> MGGIMQLVSTGYQDVFLTGDPTRSLWKRIMARKTNFAIESIETVFDVLYGSTSFINIKKAGDLLKSCVLEITMKRTSTESFYPAEQFIKSLTLLIGDQEVEKIQDFPTWSRVHDELFNDTEM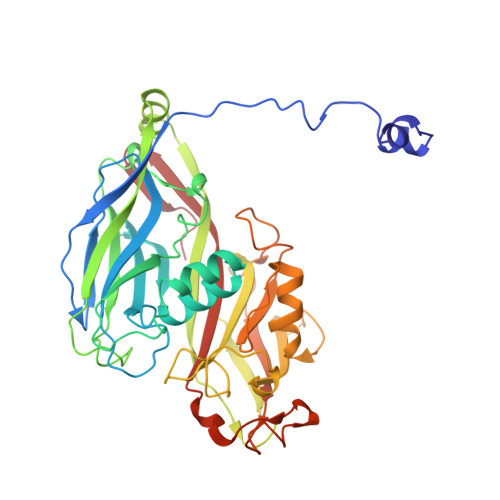RSANYRMLNFRPDDPPGAIRTFYLDLPLFFTRYLSNSLPLVALQYHEVKLKIDFEPPYNIPGIDSTYMPQVRFYGDYVFLDKPERVYFAQTEHEYIIEQLQTFVTIPNMSNSVNTTMVDLPFTLPSRYIIWVYKTNLHGQYTTSNSTFVTNEGYAPLQSAVIKCNGTDRFSERPGGYFNMVQTTQALGQAPSCGIYMYSFGVNADKQDPEGTLNFSKLDMVTLSYTNKAATAADISQVFDLSTTLENGITKFKNITIFSKNFNVLRIVEGQGGILFSN> TGGAAACAGACTGTCAGATG;> CACTGACTCATGCTCATCTG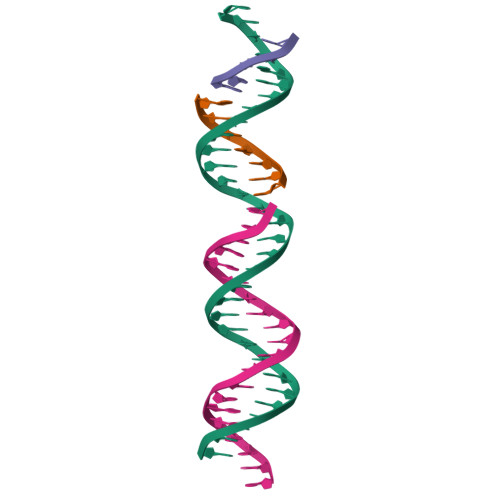ACAGTCTGTTTC;> AGCATGA;> GTCAG>GSMAPAGVPENTSLENIPVIVSKCREAFNDDANRDLKKRKQVLRSLLNLVEENTDEFCKAIHRDRRRHRDETVVMEILPLRNEVWHLIEHMDEYVKPVKPTMEGAAALDDCELQYEPLGVVLVIGTWNYPLLLILQPLLGALAAGNTAVIKPSELAPATAELLTKLLPKYVSSDVVGIVNGGVSETTAVLKERFDHILYTGSARVAEIVMAAAAKHLTPVTLELGGKSPVVVDDTCADNMKVVAERIMWGKIINAGQTSIAPDYVVVEKSMESVLVDALAEARKAMLGDKFLKVLKGELLVKQKQQFLEESDYPRIVNASHFQRLMEFMKGGKVAVGGEADEATLTIAPTILTNIDPTHPVMQEEIFGPILPVLTYENEKDILKIINSREKPLALYVFSNNKRFIRGVESRTSSGAVVVNDVVVHAGADGLPFGGVGRSGMGAYHGRYSFETFSHRRPVMRRGFLFSSIDTVRFPPYTTAK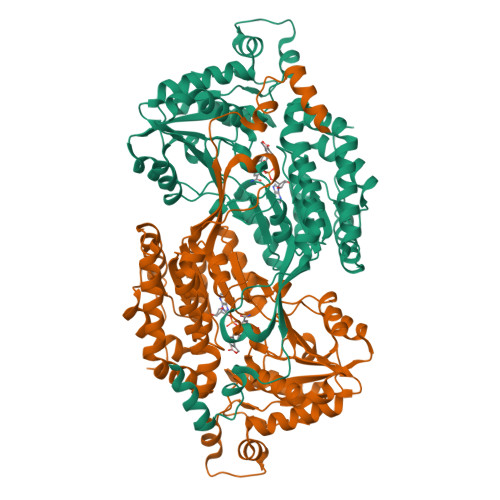SRVLNSLLKPSAEVAGAVGRSVWGVAALARVVEVGYHYMRFLMAGETTPAPSSSEPFSKSPRSNE[2x]>MARGKQNSN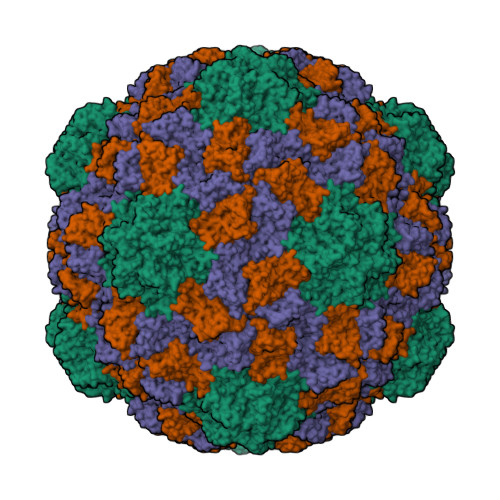QIQNNSNANGKRRKRNRRNRNPQTVPNFNPIVAKPTVAPLQTNIRSARSDVNAITVLNGSDFLTTVKVRGSNNLIDSKSRILVKQPISASSFLGTRISGLSQFWERYRWHKAAVRYVPAVPNTLACQLIGYIDTDPLDDPNVILDVDQLLRQATSQVGARQWNFSDTTTIPLIVRRDDQLYYTGQDKENVRFSQQGVFYLLQVTTLLNISGEAITNDLISGSLYLDWVCGFSMPQINPSPVEVSQLTYNADTIGNWVPPTELKQTYTQDITGLKPNSKFIIIPYMDRVSSEVLQKCTITCNEVDAVGSISYSDTSAIKCDGYILFQANSIGEATFTLVTDYQGAVDPKPYQYRIIRAIVGNN[3x]>[8x]MATKDLPTHLSSNTGFGKHHGKTQSHMAFENASTSVAASQMRNALNALAETVPDPNERKRFEAEMDNFFALFRRFLNDKAKGNVVNWDRIAPPQPSQVVNYDDIGKESSVEFLNKLAVVKLNGGLGTSMGCVGPKSVIEVREGMSFLDLSVRQIEHLNRTYNVNVPFVLMNSFNTDQDTQSIIKKYQGHNVDIITFNQSRYPRIIKDSLLPAPKSFDAPLQDWYPPGHGDVFESLYNSGTLDKLLERGVEYIFLSNADNLGAVVDTRILQHMIDTKAEYIMELTDKTKADVKGGTIIDYEGKVRLLEIAQVPKEHVNEFKSIKKFKYFNTNNIWMNLRAIKRVVEENELEMEIIANEKSIPADKKGEADQAIYQLETAVGAAIRHFKNAHGVNVPRRRFLPVKTCSDLLLVKSDLYRLEHGQLVMDPNRFGGVPVIKLGSDFKKVSDFQKRIPSIPRIVELDHLTITGAVNLGRNVTLKGTVIIVATEGSTIDIPPGSVLENCVVQGSLRILEH

UDP (uridine diphosphate)-glucose pyrophosphorylase (UGP) is a central enzyme in the metabolism of carbohydrates that catalyzes the biosynthesis of UDP-glucose, a key precursor of fungal cell wall polysaccharides. UGPs catalyze the interconversion of UTP and Glc-1-P to UDP-Glc and PPi in a Mg2+-dependent reaction, following an ordered sequential Bi-Bi mechanism in which the uridine compound is the first to enter and the last to exit the active site. In this study, we demonstrate that in A. nidulans, galF (FungiDB ID AN9148) is an essential gene encoding a UTP-specific UGP, referred to as AnUGP, a central enzyme in the metabolism of carbohydrates and assembly of the cell wall. Each AnUGP subunit (57.6 kDa protein; 514 amino acids) is composed of three domains: (i) the α-helical N-terminal (NT) domain (residues 1–81, 199–227, 354–376), (ii) the catalytic glycosyltransferase A-like (GT-A-like) domain [residues 82–198, 228–353, 377–404 (29 - 31)] containing the active site, and (iii) the C-terminal (CT) oligomerization domain (residues 405–514) containing a left-handed parallel β-helix (LβH; residues Leu461–His514).

Endogenous native AnUGP was purified owing to its ability to bind a Ni-NTA affinity column without any added tag. To take advantage of the particle’s apparent symmetry and increase the resolution of the cryoEM map, we refined the data while applying D4 symmetry, resulting in a 3.98 Å structure. Afterward, a restrained local refinement, focusing on this single subunit, yielded a 3.5 Å cryoEM map for the AnUGP monomer with local resolution ranging from 3.0 to >6 Å. Accordingly, we present a model for residues 32–82, 86–361, and 371–514 of AnUGP. Overall, cryoEM analysis of native AnUGP in solution indicates it is a homoctamer with pseudo-D4 symmetry broken by flexibility between the CT oligomerization domains and the central catalytic domains. Octameric AnUGP can be described as a tetramer of homodimers held together by two interfaces on the CT LβH, which is built of short β-strands (β17–β23) oriented parallel to each other and describing a triangular prism. The cryoEM map of the LβH region shows high local resolution (up to 3.2 Å), allowing the oligomerization interface to be described. Two AnUGP subunits build the homodimer through “end-to-end” contacts between their C-terminal extended β-strands, forming an extended intermolecular β-sheet and a joint β-helix (Fig. 3C through E, I, K). The UDP-Glc binding site faces toward the inner cavity of the complex with four pockets each in both the upper and lower rings. AnUGP displays a strong preference for UTP and, accordingly, in the structure, it is evident that the presence of small residues, Gly123 and Gly124, in the NB loop is vital for reducing steric clashes with the uridine moiety.>SIDNCAVGCPTGGSSKVSIVRHAYTLNNNSTTKFANWVAYHITKDTPASGKTRNWKTDPALNPADTLAPADYTGANAALKVDRGHQAPLASLAGVSDWESLNYLSNITPQKSDLNQGAWARLEDQERKLIDRADISSVYTVTGPLYERD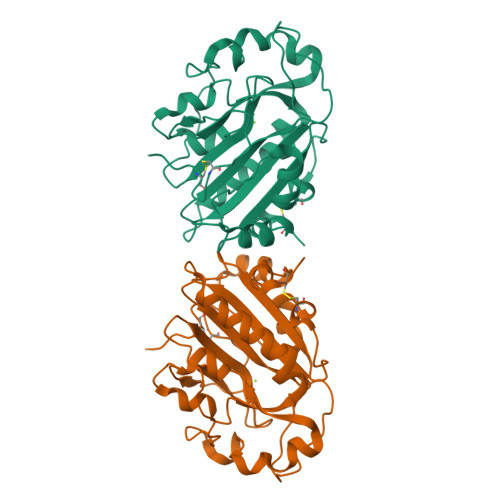MGKLPGTQKAHTIPSAYWKVIFINNSPAVNHYAAFLFDQNTPKGADFCQFRVTVDEIEKRTGLIIWAGLPDDVQASLKSKPGVLPELMGCKN[2x]>GSMASSSTAYYLKDAGFHIRNIPKAWNDWNLFHVFQNFGKVSYCRVVGQSNDGQVQLGFVNMMSVADADEVRKNMNDGNLIGENFTLKVTDHKN[2x];>[2x]MEGDIHMQENMLKISGYPGMLNTFGIAQLLTPYRVNGITMTGAQSAVVALENKFQVYQAVQDFNGKKLDRNHKLQVS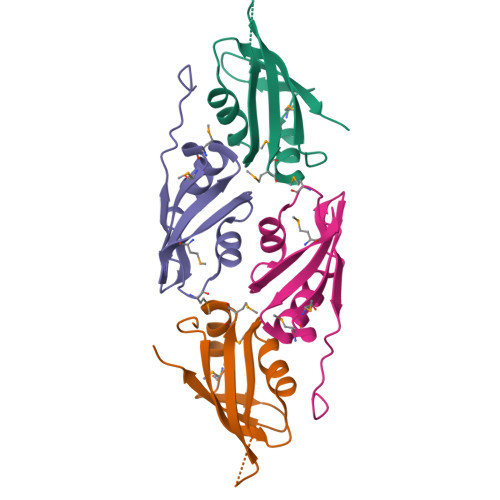SLVVSSPAVPLE>MGSSHHHHHHSSGLVPRGSMSEQYWRFKLMTEGGCNQNEATRLITVLKRKLKPFPEESINKLFENDNFCNRLSSYMAYGFGAAEEWIKKQQILSNIQPLTSEQRVDITPEKDTVSDNKPNIFGAAITFGKSPVVKLLKQNAREICESILMDEPNLKQVEYI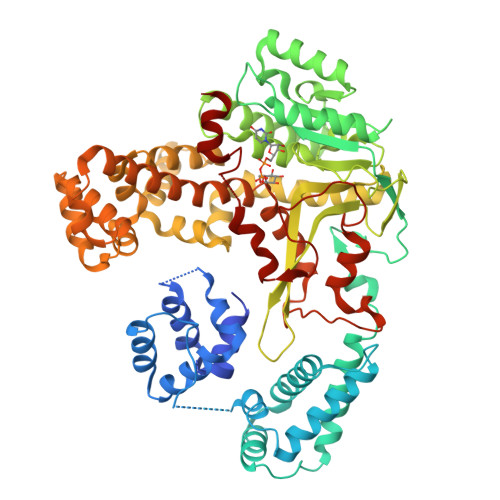FRLLALQVQETYSGEQAEKLYECIRDKKPIPSKFEEILLPIVNRIKENHTEILNESKRNHLGVTIQLNDPYSFSTKNSFCIWFSNNPNSAMPKKIKDILEERAKQNAPGVTKLVYSRACLTKKENTNFVQWAKENGITLLDFDELKCQGEDLELWNLAQAELKAMREGKGGNPAAASDLVRWISGVIGDVPIAYVDADMPMLTGNKSIKSEEVYAGHPVLLNMGSALVKDGVNLPMENVAFNTDIINFTGECKDRSIAIKRIAQSLIGNYLHVTERISKSGNPELKRLGLMPGYHQLLKDCEENNNKLSLPMLRKALTQAHSNLSSYVRFIGVQRFAEMVGAPEDAPLFQEALQQGNTIVLTNALVAYLVHGMDNVSRLNSSEKENLIKKYLGTQLSLLYKPLVMEFSGPCAVTREILPLLPTGEPTRYIENLKQPDAQILRVLQTHACVAGKTNFTSDNIPNWITSSEEVERTQSLRTDGLSWMPSEQARLSK[2x]> GPGSSRWSKDYDVCVCHSEEDLVAAQDLVSYLEGSTASLRCFLQLRDATPGGAIVSELCQALSSSHCRVLLITPGFLQDPWCKYQMLQALTEAPGAEGCTIPLLSGLSRAAYPPELRFMYYVDGRGPDGGFRQVKEAVMRYLQTLS

Mal, which is also identified as the TIR domain-containing adaptor protein (TIRAP), is essential for the TLR4 and TLR2 signaling pathways. Mal acts as a bridge adaptor to recruit the MyD88 molecule to the activated TLR4 dimer on the plasma membrane. The C-terminus (residues 80–221) of Mal, referred to as Mal-TIR, is the TIR domain and is required for interactions with TLR4, TLR2 and MyD88. The overall structure of Mal-TIR consists of a central five-stranded parallel sheet (βA-βE) surrounded by four helices (αA, αC-αE) on both sides.

The crystal structure of human Mal-TIR (residues 79–221) was determined at a resolution of 2.4 Å using the single wavelength anomalous dispersion method. The protein crystals were found to belong to the space group P43212 and to contain one molecule per asymmetric unit. In comparison with the TIR domain of MyD88, Mal-TIR has an unusually long AB loop (residues 109–129) and lacks the αB helix and the BB loop. The crystals of Valkov et al. were obtained in a solution containing 10–12% PEG 10,000, 5% PEG 3,350, 0.2 M NaCl, 0.1 M Tris-HCl (pH 7.3), and 20 mM DTT and diffracted to 3.0 Å resolution, while the crystals for this study were grown in n-cyclohexyl-2-aminoethanesulfonic acid (CHES) (pH 9.5), 150–300 mM NaCl, 10–20% glycerol and 10 mM DTT and diffracted to 2.4 Å resolution. Both structures of Mal-TIR identified the unusually long AB loop instead of the helix αB and BB loops in other known TIR domains and included two disulfide bonds (residues C89–C134 and C142–C174) and an additional DTT molecule that linked two cysteine residues, Cys91 and Cys157. Based on our Mal-TIR crystal structure, two possible interfaces (green-magenta, referred to as the symmetric dimer; green-yellow, referred to as the asymmetric dimer) mediate Mal homodimerization. The buried surface area, calculated by AREAIMOL, is 700 Å2 for the symmetric dimer and 500 Å2 for the asymmetric dimer. The interactions within the interface of the symmetric dimer primarily involve residues of the αC′ and αD helices of both monomers. Our results showed that the W156A and Y159A mutations located within the interface of the symmetric dimer caused a significant loss of Mal homodimer formation, while mutants D87A and R192A did not affect homodimer formation, indicating that the symmetric dimer observed in the crystal structure is related to the Mal homodimer formed in solution. In this dimer, the AB loops of the two molecules are oriented in opposite directions, facilitating direct interaction with TLR4 and MyD88. We conclude that the AB loop of Mal-TIR plays an important role in TLR signaling through interacting with TLR4 and MyD88 simultaneously.> MEQRETIMLPGSDYNHWLIVMEFPKDPAPSRDQMIDTYLNTLATV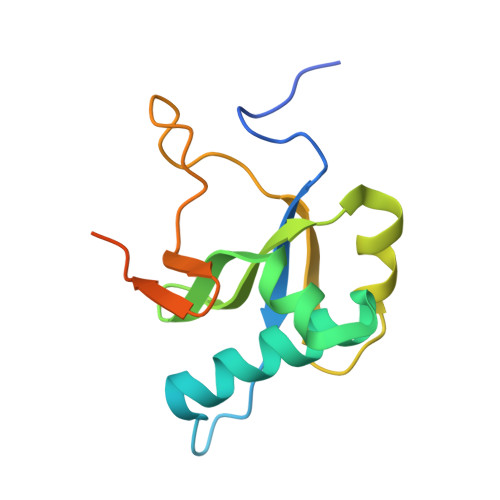LGSMEEAKKNMYAFSTTTYTGFQCTIDEETSEKFKGLPGVLWVLPDSYIDVKNKDYGGDKYINGEIIPSTYPTYQPKQLEHHHHHHHH3-(7-ethoxynaphthalen-2-yl)-1-(2-methylpropyl)-1H-pyrazolo[3,4-d]pyrimidin-4-amine | C21 H23 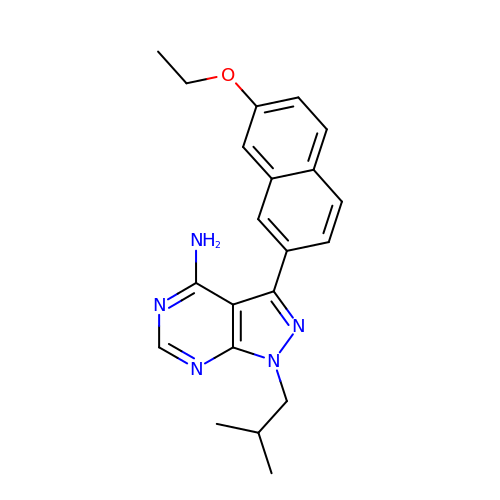N5 O | AEVLTZJWDLNUCI-UHFFFAOYSA-N> MLPRETDEEPEEPGRRGSFVEMVDNLRGKSGQGYYVEMTVGSPPQTLNILVDTGSSNFAVGAAPHPFLHRYYQRQLSSTYRDLRKGVYVPYTQGKWEGELGTDLVSIPHGPNVTVRANIAAITESDKFFINGSNWEGILGLAYAEIARPDDSLEPFFDSLVKQTHVPNLFSLQLCGAGFPLNQSEVLASVGGSMIIGGIDHSLYTGSLWYTPIRREWYYEVIIVRVEINGQDLKMDCKEYNYDKSIVDSGTTNLRLPKKVFEAAVKSIKAASSTEKFPDGFWLGEQLVCWQAGTTPWNIFPVISLYLMGEVTNQSFRITILPQQYLRPVEDVATSQDDCYKFAISQSSTGTCMGAVIMEGFYVVFDRARKRIGF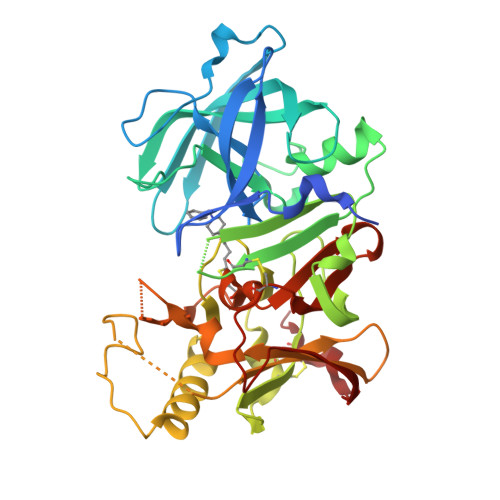AVSACHVHDEFRTAAVEGPFVTLDMEDCGYN(3R,4R)-1-METHANESULFONYL-PYRROLIDINE-3,4--DICARBOXYLIC ACID 3-[(3-FLUORO-4-METHOXY-PHENYL)-AMIDE] 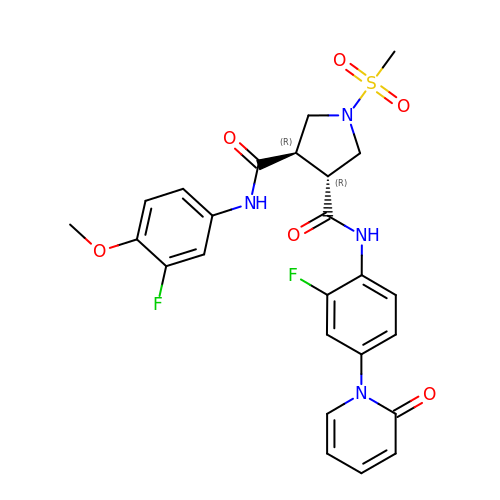4-{[2-FLUORO-4-(2-OXO-2H-PYRIDIN-1-YL)-PHENYL]-AMIDE} | C25 H24 F2 N4 O6 S | JORQWQCWRYRBEL-ROUUACIJSA-N> MRHERVVIIKNMFHPMDFED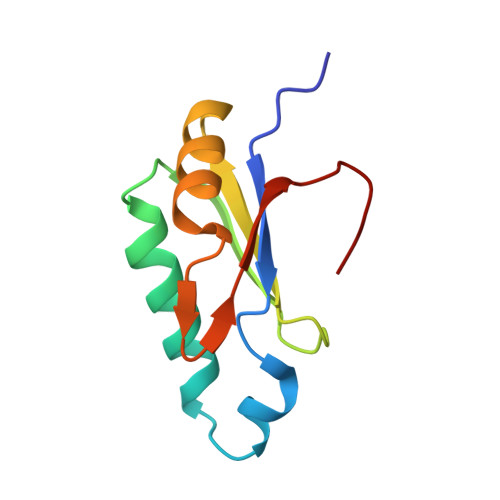DPLVLNEIREDLRVECSKFGQIRKLLLFDRHPDGVASVSFRDPEEADYCIQTLDGRWFGGRQITAQAWDGTTDY>IEEEEKKPRVKDTVIREHNKWILKKIRFQGNLNTKKMLNPGKLSEQLDREGRKRNIYNHQIGTIMSSAGIRLEKLPIVRAQTDTKTFHEAIRDKIDKSENRQNPELHNKLLEIFHTIAQPTLKHTYGEVTWEQLEAGVNRKGAAGFLEKKNIGE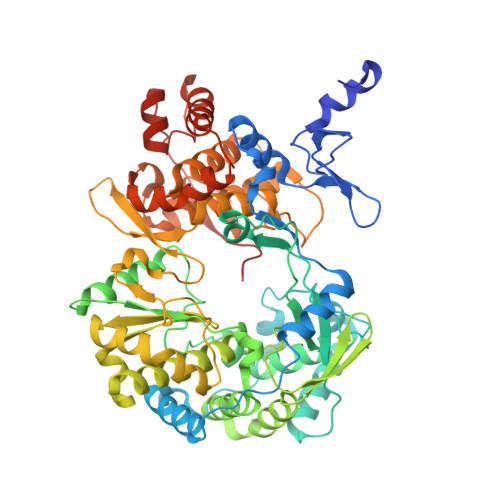VLDSEKHLVEQLVRDLKAGRKIKYYETAIPKNEKRDVSDDWQAGDLVVEKRPRVIQYPEAKTRLAITKVMYNWVKQQPVVIPGYEGKTPLFNIFDKVRKEWDSFNEPVAVSFDTKAWDTQVTSKDLQLIGEIQKYYYKKEWHKFIDTITDHMTEVPVITADGEVYIRNGQRGSGQPDTSAGNSMLNVLTMMYAFCESTGVPYKSFNRVARIHVCGDDGFLITEKGLGLKFANKGMQILHEAGKPQKITEGEKMKVAYRFEDIEFCSHTPVPVRWSDNTSSHMAGRDTAVILSKMATRLDSSGERGTTAYEKAVAFSFLLMYSWNPLVRRICLLVLSQQPETDPSKHATYYYKGDPIGAYKDVIGRNLSELKRTGFEKLANLNLSLSTLGVWTKHTSKRIIQDCVAIGKEEGNWLVKPDRLISSKTGHLYIPDKGFTLQGKHYEQLQL[4x]>[4x]GPMDPDTNLLKNVILEILSIEPDLYKQSSIVDDPYKLAMSAIRLRATIHELNCCRDLGIIHNTKEISLNMVIDRAIPIHPTFQHIVPDGYTIDRANMTIIVLEASTRSMPSDQKRKITSDKLKYSGVEDHLKHEGWLFNIIVISETKPRNGNVPERLLFELLKLSLSILSYSDKSSQWISEEEYDELKRSLTTYDFKTLTSEFSGTK

The two genome segments code for four viral proteins, the nucleoprotein (NP), the glycoprotein-precursor, the small matrix protein Z and the large > 200 kDa L protein which harbors the viral RNA-dependent RNA polymerase. The L protein synthesizes two distinct RNA species: (i) the antigenomic and genomic RNA as products of genome replication and (ii) the shorter capped viral mRNAs during transcription. To initiate viral transcription, the L protein presumably uses a process called cap-snatching. It is assumed that the L protein cleaves host cell mRNAs downstream of the 5'-cap structure and uses this short capped RNA as a primer for viral mRNA synthesis. Here we present the crystal structures of the two terminal domains of the CASV L protein: the cap-snatching endonuclease in the N-terminus and the 326 C-terminal residues, which, by analogy to LASV, might play a role in transcription.

Therefore, we expressed and purified the first 205 residues of the CASV L protein as N-terminally His-tagged protein. As expected from the metal-dependent enzymatic mechanism of viral endonucleases, thermal stability assays showed a concentration dependent stabilization of the protein by manganese ions with an increase in melting temperature of up to ~10°C at a concentration of 10 mM manganese (protein concentration in the assay 4.2 μM). After His-tag cleavage, the protein was crystallized and the crystals diffracted to a resolution of 1.9 Å. The native protein crystallized in space group P212121 with four molecules per asymmetric unit. The structures of the four molecules are very similar with the only difference in the C-terminal 15 residues, which are not visible in all molecules (RMSD between 0.227 and 0.317 Å). The CASV endonuclease has basically the same fold as endonucleases from LASV, Pichinde virus (PICV), and lymphocytic choriomeningitis virus (LCMV) even though the amino acid sequence of this protein is hardly conserved among these viruses (identity ranging between 20 and 55% and similarity ranging between 54 and 79%). Slight differences between the structures were observed in the long α-helix parallel to the β-sheet (α-helix shown in orange), which is separated into two helices in CASV endonuclease domain compared to the other structures, as well as in the helical region shown in green, which is composed of four to six helices of different length and orientation. The highly conserved residues of the endonuclease active site are positioned as in other arenavirus endonuclease structures. We also tested for endonuclease activity using our previously established RNA cleavage assay, however, we did not observe enzymatic activity of the isolated domain.>[2x]MTTVIDATMAYRFLEEATDSSSSSSSSKLESSPVDAVLFVGMSLVLGIASRHLLRGTRVPYTVALLVIGIALGSLEYGAKHNLGKIGHGIRIWNEIDPELLLAVFLPALLFESSFSMEVHQIKRCLGQMVLLAVPGVLISTACLGSLVKVTFPYEWDWKTSLLLGGLLSATDPVAVVALLKELGASKKLSTIIEGESLMNDGTAIVVFQLFLKMAMGQNSDWSSIIKFLLKVALGAVGIGLAFGIASVIWLKFIFNDTVIEITLTIAVSYFAYYTAQEWAGASGVLTVMTLGMFYAAFARTAFKGDSQKSLHHFWEMVAYIANTLIFILSGVVIAEGILDSDKIAYQGNSWRFLFLLYVYIQLSRVVVVGVLYPLLCRFGYGLDWKESIILVWSGLRGAVALALSLSVKQSSGNSHISKETGTLFLFFTGGIVFLTLIVNGSTTQFVLRLLRMDILPAPKKRILEYTKYEMLNKALRAFQDLGDDEELGPADWPTVESYISSLKGSEGELVHHPHNGSKIGSLDPKSLKDIRMRFLNGVQATYWEMLDEGRISEVTANILMQSVDEALDQVSTTLCDWRGLKPHVNFPNYYNFLHSKVVPRKLVTYFAVERLESACYISAAFLRAHTIARQQLYDFLGESNIGSIVINESEKEGEEAKKFLEKVRSSFPQVLRVVKTKQVTYSVLNHLLGYIENLEKVGLLEEKEIAHLHDAVQTGLKKLLRNPPIVKLPKLSDMITSHPLSVALPPAFCEPLKHSKKEPMKLRGVTLYKEGSKPTGVWLIFDGIVKWKSKILSNNHSLHPTFSHGSTLGLYEVLTGKPYLCDLITDSMVLCFFIDSEKILSLQSDSTIDDFLWQESALVLLKLLRPQIFESVAMQELRALVSTESSKLTTYVTGESIEIDCNSIGLLLEGFVKPVGIKEELISSPAALSPSNGNQSFHNSSEASGIMRVSFSQQATQYIVETRARAIIFNIGAFGADRTLHRRPSSLTPPRSSSSDQLQRSFRKEHRGLMSWPENIYAKQQQEINKTTLSLSERAMQLSIFGSMVNVYRRSVSFGGIYNNKLQDNLLYKKLPLNPAQGLVSAKSESSIVTKKQLETRKHACQLPLKGESSTRQNTMVESSDEEDEDEGIVVRIDSPSKIVFRNDL

Salt-overly-sensitive 1 (SOS1) is a unique electroneutral Na+/H+ antiporter at the plasma membrane of higher plants and plays a central role in resisting salt stress. SOS1, which is highly conserved in the phylae of the plant kingdom, is identified as the only Na+/H+ transporter that localizes at the plasma membrane and specifically exports Na+ by utilizing the electrochemical proton gradient generated by H+-ATPase6,7. SOS1 forms a homodimer and is composed of a TMD and an intracellular domain. Previous studies have shown that the C-terminus of SOS1 contains an autoinhibitory domain to keep the transporter in a resting state with basal activity.

We firstly focused on the 2.8-Å resolution SOS1-ClassII to display structural features of SOS1 and name SOS1-ClassII as SOS1 in short. The resulting dimeric SOS1 is approximately 85 Å in length, 95 Å in width, and 120 Å in height. Nevertheless, the transport activity of SOS1 was eliminated by the D201A mutation, even in the presence of the SOS2-SOS3 complex, substantiating the significance of the D201TM6 in cation association in both inward-facing and outward-facing conformations. Strikingly, in the current SOS1 structure, D201TM6 is approximately 5 Å away from the apex of the intracellular cavity and is not accessible by the solvent, indicating that the structure is stabilized in an occluded state, which prevents ion binding and thus inhibits the transporter. To understand the molecular basis of the inaccessibility of D201TM6, we compared the core domains of SOS1 and NHE1-CHP1 in the inward-facing conformational (NHE1-CHP1IF) state, giving rise to an RMSD of 1.60 Å over 180 Cα atom pairs. However, TM5b exhibits a dramatic local conformational change, being displaced by 5 Å toward the dimerization domain compared with that of the NHE1-CHP1IF complex. Consequently, D201TM6 is completely buried in a cavity composed of TM3, TM5b, and TM10 and cannot interact with ions from the intracellular side. Strikingly, TM5b assumes a conformation similar to that of the NHE1-CHP1OF complex, indicating that SOS1 may be trapped in an occluded state, an intermediate state between inward- and outward-facing conformational states. The C-loop is closely embedded in a cavity formed by the HC1, HC3, and HC5 helices from the α-CTD of the same subunit, mediated by hydrophobic and electrostatic interactions. The C-helix is located underneath the α-CTD and grips CNBLD from the same subunit and α-CTD from another subunit with extensive contact interfaces, thus stabilizing the dimerization of SOS1 and a specific geometry between α-CTD and CNBLD. Taken together, the results show that C-loop and C-helix are involved in extensive intramolecular or intermolecular interactions with α-CTD and CNBLD and presumably stabilize the intracellular domain in a specific conformation to inhibit SOS1 activity.> GMRRELA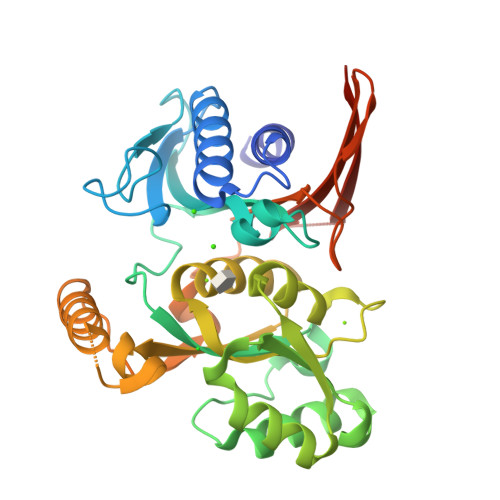IEFSRVTESAALAGYKWLGRGDKNTADGAAVNAMRIMLNQVNIDGTIVIGEGEIAEAPMLYIGEKVGTGRGDAVDIAVDPIEGTRMTAMGQANALAVLAVGDKGCFLNAPDMYMEKLIVGPGAKGTIDLNLPLADNLRNVAAALGKPLSELTVTILAKPRHDAVIAEMQQLGVRVFAIPDGDVAASILTCMPDSEVDVLYGIGGAPEGVVSAAVIRALDGDMNGRLLARHDVKGDNEENRRIGEQELARCKAMGIEAGKVLRLGDMARSDNVIFSATGITKGDLLEGISRKGNIATTETLLIRGKSRTIRRIQSIHYLDRKDPEMQVHIL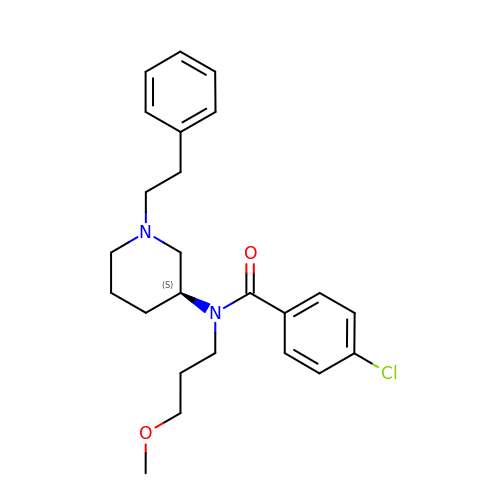4-chloro-N-(3-methoxypropyl)-N-[(3S)-1-(2-phenylethyl)piperidin-3-yl]benzamide | C24 H31 Cl N2 O2 | OOUGHDJEJNMXSV-QHCPKHFHSA-N> GHMKITVRGSEMVYPAAETPRRRLWNSGPDLVVPRFHTPSVYFFRRRDGEGNDLAAAD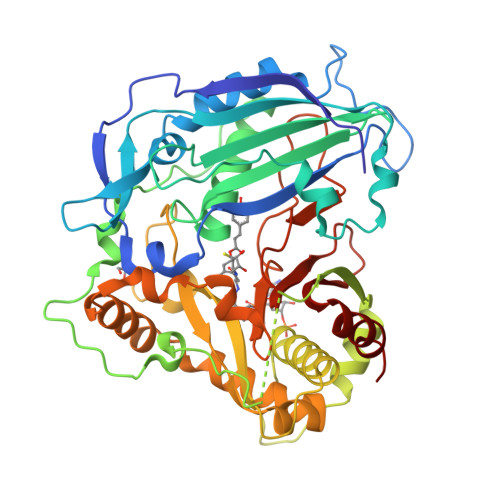GSFFDGARMRRALAEALVPFYPMAGRLARDEDGRVEIDCNAGGVLFQEADAPDATVDDFGDFAPTMELKRLIPTVEYTDDISAFPLLVVQVTHFKCGGVAIGVGMQHHVADGFSGLHFINSWADLCRGVPFAVMPYIDRSLLRARDPPTPVYPHVEYQPAPAMLSEPPQAPLMAKPATPPAAVAIFRLSRADLGRLRSQIPAREGVPRLSTYAVLAAHVWRCASLARGLPADQPTKLYCATDGRQRLQPPLPEGYFGNVIFTATPLADAGTVTAGVAEGAAVIQAALDRMDEGYCRSALDYLELQPDLSALVRGAHTFRCPNLGLTSWVRLPIHDADFGWGRPVFMGPGGIAYEGLAFVLPSANRDGSLSVAISLQAEHMEKFRKFIYDF Several natural systems exhibit ‘facilitated dissociation’, in which an effector (E) can bind to a target–host (TH) complex to form an excited ternary complex (THE)20–26 from which the target dissociates quickly. We set out to design protein systems that undergo facilitated dissociation. We use a switchable target binder (host) and a flexible effector that can rapidly bind to and switch the target–host complex to induce a large steric clash with the target, forming a strained excited ternary complex. We show here that by explicitly considering excited intermediate states when designing coupled protein systems, a broad range of facilitated dissociation systems can be designed.

To investigate the mechanism of facilitated dissociation, we focused on AS1, the design with the tightest effector binding (Kd,H:E ≈ 10 pM). We used X-ray crystallography to structurally characterize multiple states of our designed systems. For both the AS1 and the AS5 systems, the crystal structures of the hosts alone and of the host–effector complexes closely match the design models (maximum 1.3 Å Cα root mean square deviation (RMSD)). The unbound structures show an open hydrophobic cleft in the new designed state X poised to bind the effector, and the effector-bound structures show that binding the effector causes the two switch domains to register-shift into the designed state Y. Starting from AS0, we constructed a new state X by shifting the two domains from their state Y positions relative to each other (by one heptad along the helix of domain 1 that contacts domain 2), building a new loop between the domains, and optimizing single sequences that could adopt both this new state X and the original effector-bound state Y. This approach maintains the open cleft in state X by introducing minimal rotation from state Y and simplifies the multi-state sequence-design challenge by minimizing the local structural differences between the two states. Transition between conformational states occurs by a register shift throughout which the cleft could remain open and bind the effector.

> MSGSMKEEIKRLAEELKEKTKNEEIKRLAEEAAELAERSDDPEVLEVVKKALEEALKSKNEEKIELLLLVAVLVAEAGSVDAVEEKLEIALLALKLAEESKDPRIIRGALRAAIAALRSDDPLALKTVKEALERARASKDERLIRAILAAAYAFALLAVAGASAERLKEAEAIVKELIAAAEKGASPQELVLLVIEMMVKGMGVTMETHRSGNEVKVVIKGLHESQQEVLLEAVLFAAELMGVRVRIRFKGDTVTIVVREGSGS> MLPRLICINDYEQHAKSVLPKSIYDYYRSGANDEETLADNIAAFSRWKLYPRMLRNVAETDLSTSVLGQRVSMPICVGATAMQRMAHVDGELATVRACQSLGTGMMLSSWATSSIEEVAEAGPEALRWLQLYIYKDREVTKKLVRQAEKMGYKAIFVTVDTPYLGNRLDDVRNRFKLPPQLRMKNFETSTLSFSPEENFGDDSGLAAYVAKAIDPSISWEDIKWLRRLTSLPIVAKGILRGDDAREAVKHGLNGILVSNHGARQLDGVPATIDVLPEIVEAVEGKVEVFLDGGVRKGTDVLKALALGAKAVFVGRPIVWG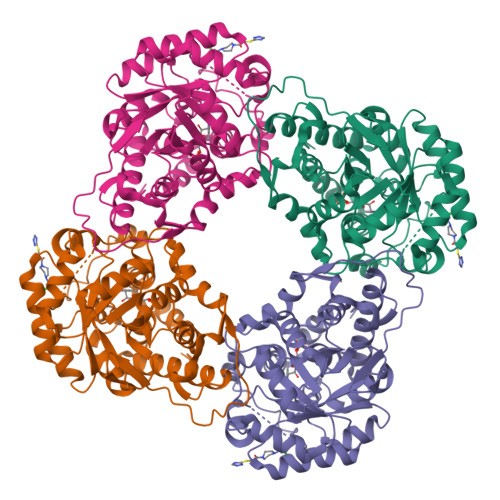LAFQGEKGVQDVLEILKEEFRLAMALSGCQNVKVIDKTLVRK>[2x]ARTFFVGGNFKLNGSKQSIKEIVERLNTASIPENVEVVICPPAT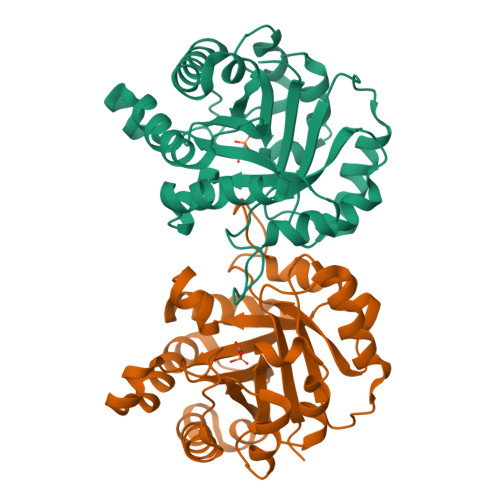YLDYSVSLVKKPQVTVGAQNAYLKASGAFTGENSVDQIKDVGAKWVILGHSERRSYFHEDDKFIADKTKFALGQGVGVILCIGETLEEKKAGKTLDVVERQLNAVLEEVKDWTNVVVAYEPVWAIGTGLAATPEDAQDIHASIRKFLASKLGDKAASELRILYGGSANGSNAVTFKDKADVDGFLVGGASLKPEFVDIINSRN>MKSLTYFWLFLPVLSTLSLPQDVTRCSAKTNFRRFFSKFNVQAPAVVVLGGYLPIGENQGVNSTWYCAGQHPTASGVHGIFVSHIRGGHGFEIGISQEPFDPSGYQLYLHKATNGNTNATARLRICQFPSIKTLGPTANNDVTIGRNCLFNKAIPAHMSEHSVVGITWDNDRVTVFSDKIYYFYFKNDWSRVATKCYNSGGCAMQYVYEPTYYMLNVTSAGEDGISYQPCTANCIGYAANVFATEPNGHIPEGFSFNNWFLLSNDSTLVHGKVVSNQPLLVNCLLAIPKIYGLGQFFSFNQTIDGVCNGAAVQRAPEALRFNINDTSVILAEGSIVLHTALGTNFSFVCSNSSNPHLATFAIPLGATQVPYYCFFKVDTYNSTVYKFLAVLPPTVREIVITKYGDVYVNGFGYLHLGLLDAVTINFTGHGTDDDVSGFWTIASTNFVDALIEVQGTAIQRILYCDDPVSQLKCSQVAFDLDDGFYPFSSRNLLSHEQPISFVTLPSFNAHSFVNITVSASFGGHSGANLIASDTTINGFSSFCVDTRQFTISLSYNVTNSYGYVSNSQDSNCPFTLQSVNDYLSFSKFCVSTSLLASACTIDLFGYPEFGSGVKFTSLYFQFTKGELITGTPKPLEGVTDVSFMTLDVCTKYTIYGFKGEGIITLTNSSFLAGVYYTSDSGQLLAFKNVTSGAVYSVTPCSFSEQAAYVDDDIVGVISSLSSSTFNSTRELPGFFYHSNDGSNCTEPVLVYSNIGVCKSGSIGYVPSQSGQVKIAPTVTGNISIPTNFSMSIRTEYLQLYNTPVSVDCATYVCNGNSRCKQLLTQYTAACKTIESALQLSARLESVEVNSMLTISEEALQLATISSFNGDGYNFTNVLGVSVYDPARGRVVQKRSFIEDLLFNKVVTNGLGTVDEDYKRCSNGRSVADLVCAQYYSGVMVLPGVVDAEKLHMYSASLIGGMVLGGFTAAAALPFSYAVQARLNYLALQTDVLQRNQQLLAESFNSAIGNITSAFESVKEASSQTSRGLNTVAHALTKVQEVVNSQGAALTQLTVQLQHNFQAISSSIDDIYSRLDILSADVQVDRLITGRLSALNAFVAQTLTKYTEVQASRKLAQQKVNECVKSQSQRYGFCGGDGEHIFSLVQAAPQGLLFLHTVLVPSDFVDVIAIAGLCVNDEIALTLREPGLVLFTHELQNHTATEYFVSSRRMFEPRKPTVSDFVQIESCVVTYVNLTRDQLPDVIPDYIDVNKTRDEILASLPNRTGPSLPLDVFNATYLNLTGEIADLEQRSESLRNTTEELQSLIYNINNTLVDLEWLNRVETYIKWPWWVWLIIFIVLIFVVSLLVFCCISTGFCGCFGCCCACFSGCCRGPRLQPYEVFEKVHVQ[3x]

The trimeric spike (S) glycoprotein of PEDV is responsible for virus-host recognition, membrane fusion, and is the main target for vaccine development and antigenic analysis. The PEDV S consists of an S1 subunit, an S2 subunit, a transmembrane domain (TM), and a cytosolic tail. The S1 subunit can be subdivided into three domains and two subdomains, namely the domain 0 (D0), the N-terminal domain (NTD), the subdomain 1 (SD1), the C-terminal domain (CTD), and the subdomain 2 (SD2). The D0 modulates the enteric tropism of PEDV by binding to sialic acids (SAs) on the surface of enterocytes.

To obtain further insights into the structure and dynamics of the PEDV S at a higher resolution, we collected cryo-EM data from the same batch of viral particles. The particles were refined with a C3 symmetry followed by symmetry expansion to extract further information with regard to the local motions within individual protomers. The set of S trimer particles with all three protomers in the D0-down conformation was refined with C3 symmetry, resulting in a D0DDD map with a global resolution of 4.7 Å. 68% of the final S trimer particles corresponded to the D0DDD arrangement. The atomic models corresponding to the PEDV S in the D0DDD and D0UDD arrangements were built. The D0-down state has the D0 tucked against the S2 subunit, while in the D0-up state, the lifted D0 adopts a propeller-like conformation. Despite the moderate resolutions of our cryo-EM maps, we observed well-defined secondary structure elements and bulky side chains, with clear protrusions from the asparagine side chains at 21 out of 23 putative N-glycosylation sites, which we attributed as the glycan structures. In contrast, the D0-down conformation exhibited a cluster of N-glycans on Asn726, Asn873, and Asn118, which made extensive contact with the D0 and S2 subunit. Despite the discrepancy between cryo-ET and cryo-EM in terms of the absolute proportions of the individual states, it is clear that the D0-down conformation is energetically more favorable than the D0-up conformation.>[4x]MARQPYRFPQARIPERGSGVFRLTVRNAMAHRDSEMKEECLREDLKFYFMSPCEKYRARRQIPWKLGLQILKIVMVTTQLVRFGLSNQLVVAFKEDNTVAFKHLFLKGYSGTDEDDYSCSVYTQEDAYESIFFAINQYHQLKDITLGTLGYGENEDNRIGLKVCKQHYKKGTMFPSNETLNIDNDVELDCVQLDLQDLSKKPPDWKNSSFFRLEFYRLLQVEISFHLKGIDLQTIHSRELPDCYVFQNTIIFDNKAHSGKIKIYFDSDAKIEECKDLNIFGSTQKNAQYVLVFDAFVIVICLASLILCTRSIVLALRLRKRFLNFFLEKYKRPVCDTDQWEFINGWYVLVIISDLMTIIGSILKMEIKAKNLTNYDLCSIFLGTSTLLVWVGVIRYLGYFQAYNVLILTMQASLPKVLRFCACAGMIYLGYTFCGWIVLGPYHDKFENLNTVAECLFSLVNG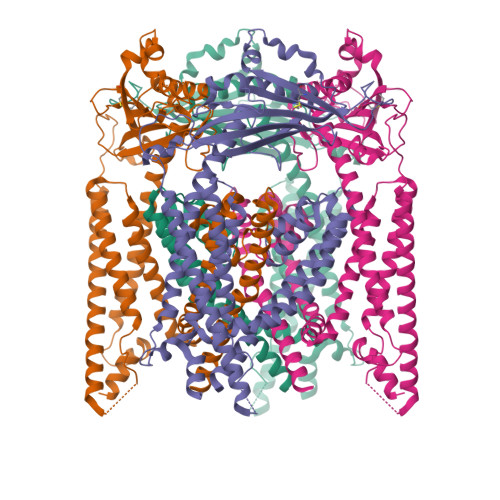DDMFATFAQIQQKSILVWLFSRLYLYSFISLFIYMILSLFIALITDSYDTIKKFQQNGFPETDLQEFLKECSSKEEYQKESSAFLSCICCRRRKRSDDHLIPIS> MENGYTYEDYKNTAEWLLSHTKHRPQVAIICGSGLGGLTDKLTQAQIFDYGEIPNFPRSTVPGHAGRLVFGFLNGRACVMMQGRFHMYEGYPLWKVTFPVRVFHLLGVDTLVVTNAAGGLNPKFEVGDIMLIRDHINLPGFSGQNPLRGPNDERFGDRFPAMSDAY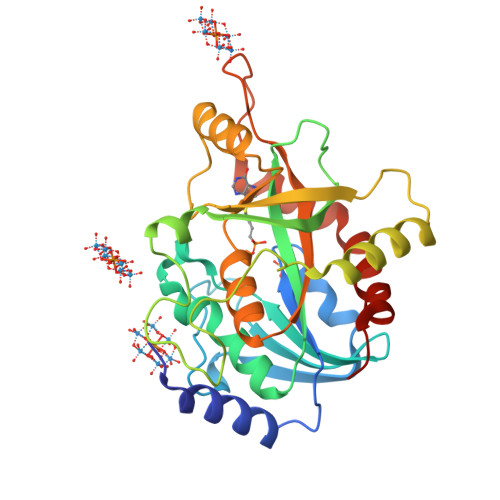DRTMRQRALSTWKQMGEQRELQEGTYVMVAGPSFETVAECRVLQKLGADAVGMSTVPEVIVARHCGLRVFGFSLITNKVIMDYESLEKANHEEVLAAGKQAAQKLEQFVSILMASIPLPDKAS> GPVGEPVASEINEASKVSSRLLTQDILFRKDRQATISLPIKLPVEDIITQTCDKITYGPLKFLDLLEKETAVLPLSTDITCPACLGRAVLVGKWECPAHVAVNESDLTVFGPNKEEHVPQFVTVQQPSDGKMQRLFFAKFLGTEESLAVLRVPGPDGHLCIQEALIHFKELSGAGVCSLWKANDSREEGLEMKQVDCLETTVLENQTCIATTLSKKIYHRLYCGERLMTGGQVSTRVLLTALGFYKRQPYTFHRVPKGMVYVHLIDSGSEDYMEYSECEEVTPGRYEDKQISYTFYTDLFQTADGEPVLASVWGTSGLKDSAYESCAFVIPTKGRRKLVPRRIMSKCYPFRLTYHPSTMT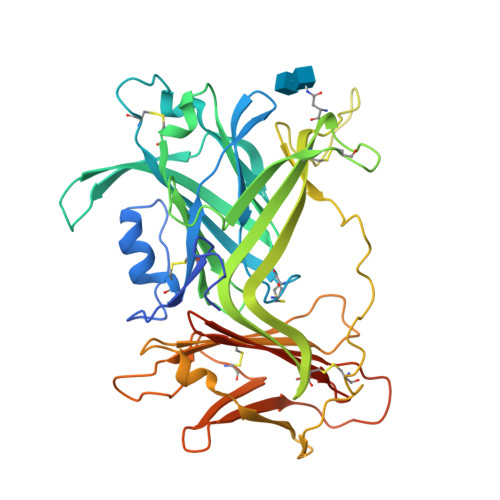VRLDVRVEKHHGATDQGFVFLKMESGTYSEGREYYLDRVLWGEDSSTNNVLQHHHHHHHH> MAAVQLSELRDRQAIFETLVAKGRELLACDRVIVYAFDDNYVGTVVAESVAEGWPQARDQVIEDPCFREHW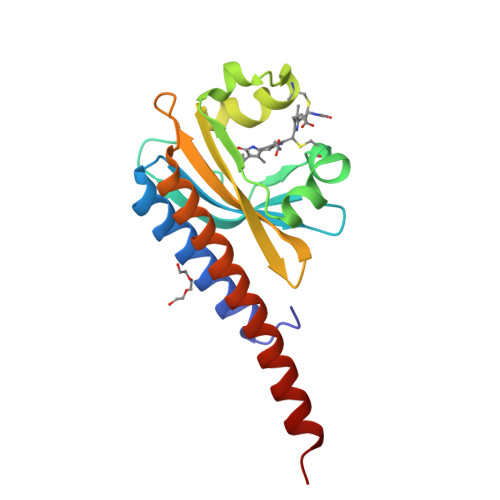VEAYRQGRIQATTDIFKAGLTECHLNQLRPLKVRANLVVPMVIDDQLFGLLIAHQASEPRQWQEIEIDQFSELASTGSLVLERLHFLEQTIASLHHHHHH> ASRYLTDFEPIQCMGRGGFGVVFEAKNKVDDCNYAIKRIRLPNRELAREKVMREVKALAKLEHPGIVRYFNAWLETPPEKWQEEMDEIWLKDESTDWPLSSPSPMDAPSVKIRRMDPFSTKNTVGQLQPSSPKVYLYIQMQLCRKENLKDWMNRRCSLEDREHGVCLHIFIQ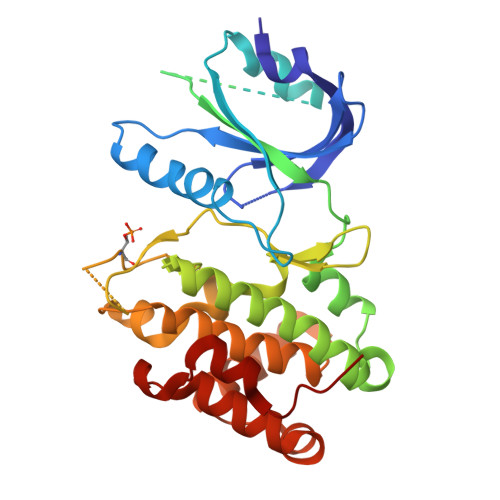IAEAVEFLHSKGLMHRDLKPSNIFFTMDDVVKVGDFGLVTAMDQDEEEQTVLTPMPAYATHTGQVGTKLYMSPEQIHGNNYSHKVDIFSLGLILFELLYSFSTQMERVRIITDVRNLKFPLLFTQKYPQEHMMVQDMLSPSPTERPEATDIIENAIFENL> MTAKQFRHGGENLAVRYALADCELGRCLVAESERGICAILLGDDDATLISELQQMFPAADNAPADLMFQQHVREVIASLNQRDTPLTLP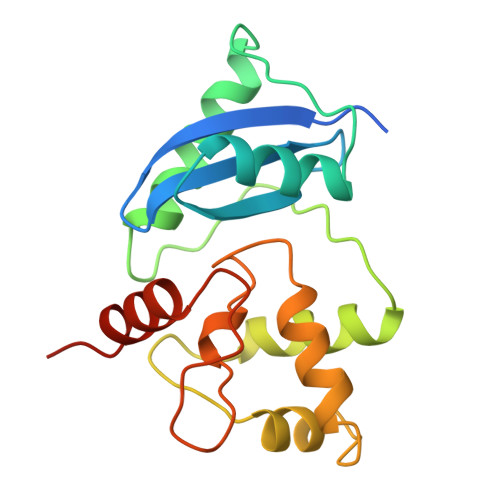LDIRGTAFQQQVWQALRTIPCGETVSYQQLANAIGKPKAVRAVASACAANKLAIVIPCHRVVRGDGSLSGYRWGVSRKAQLLRREAENEER>MCTSILYSPKDHYFGRNLDYEIAYGQKVVITPRNYEFKFANLPAEKSHYAMIGIAAVANNTPLYCDAINEKGLGVAGLSFAGQGKYFPVVEDKKNIASFEFISYILATYETVDQVKENLTDVNISDVSFSKNTPASELHWLVGDKTGKSIVVESDEKGLHVYDNPVNALTNAPLFPQQLTNLANYAAVVPGQPNNDFLPGV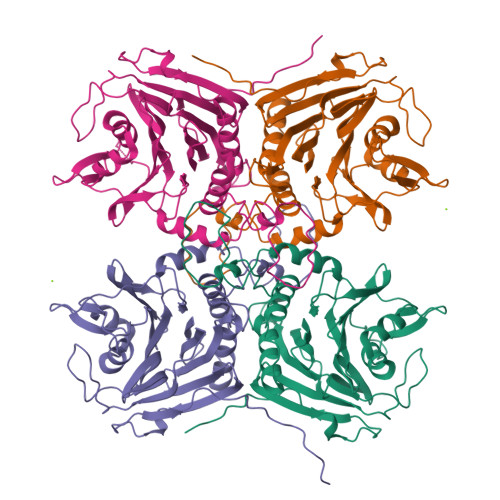DLKMYSRSLGTHHLPGGMDSESRFVKVCFALNHAPKDSDEVESVTNFFHILQSVEQVKGMDEVGPNIFEYTMYTSCMNLEKGILYFNCYDDSRISAVDMNKEDLSSSDLIVFDLFKKQDISFINHHHHHH[8x]> MILDTDYITEDGKPVIRIFKKENGEFKIDYDRNFEPYIYALLKDDSAIEDVKKITAERHGTTVRVVRAEKVKKKFLGRPIEVWKLYFTHPQDQPAIRDKIKEHPAVVDIYEYDIPFAKRYLIDKGLIPMEGDEELKMLAFDIETLYHEGEKFAEGPILMISYADEEGARVITWRNIDLPYVDVVSTEKEMIKRFLKVVKEKDPDVLITYNGDNFAFAYLKKRSEKLGVKFILGREGSEPKIQRMGDRFAVEVKGRIHFDLYPVIRRTINLPTYTLEAVYEAIFGQPKEKVYAEEIAQAWETGEGLERVARYSMEDAKVTYELGKEFFPMEAQLSRLVGQSLWDVSRSSTGNLVEWFLLRKAYERNELAPNKPDERELARRRESYAGGYVKEPERGLWENIVYLDFRSLYPSIIITHNVSPDTLNREGCEEYDVAPQVGHKFCKDFPGFIPSLLGDLLEERQKVKKKMKATIDPIEKKLLDYRQRAI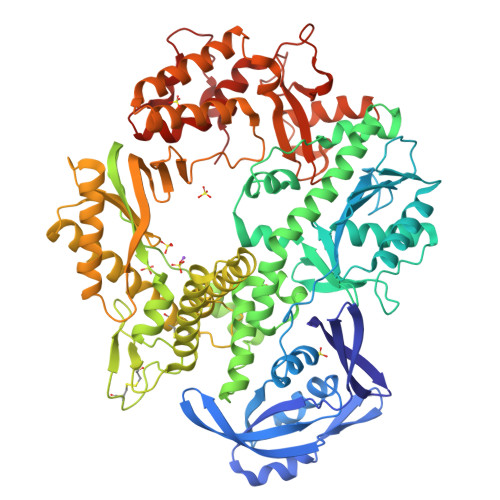KILANSFYGYYGYAKARWYCKECAESVTAWGRQYIETTIREIEEKFGFKVLYADTDGFFATIPGADAETVKKKAKEFLDYINAKLPGLLELEYEGFYKRGFFVTKKKYAVIDEEDKITTRGLEIVRRDWSEIAKETQARVLEAILKHGDVEEAVRIVKEVTEKLSKYEVPPEKLVIYEQITRDLKDYKATGPHVAVAKRLAARGIKIRPGTVISYIVLKGSGRIGDRAIPFDEFDPAKHKYDAEYYIENQVLPAVERILRAFGYRKEDLRYQKTRQVGLGAWLKPKT>[8x]MSLAQYPVIGID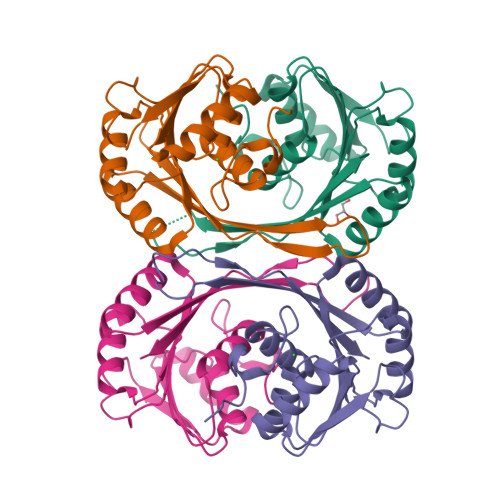DDEFATAKKLITKQEVRAVTLSKLRLQDDLVMWDIGAGSASVSIEASNLMPNGRIFALERNPQYLGFIRDNLKKFVARNVTLVEAFAPEGLDDLPDPDRVFIGGSGGMLEEIIDAVDRRLKSEGVIVLNAVTLDTLTKAVEFLEDHGYMVEVACVNVAKTKGLTEYKMFESHNPVYIITAWKSDEGHHHHHH>QVVSQGWKYFKGNFYYFSLIPKTWYSAEQFCVSRNSHLTSVTSESEQEFLYKTAGGLIYWIGLTKAGMEGDWSWVDDTPFNKVQSARFWIPGEPNNAGNNEHCGNIKAPSLQAWNDAPCDKTFLFICKRPYVPSEP[4x]

Langerhans cells are characterized by the presence of langerin (CD207), a C-type lectin that can act as a pathogen receptor by binding to surface glycoconjugates of microorganisms. Langerin has an extracellular region that contains (1) a C-type carbohydrate-recognition domain (CRD) that binds sugars and (2) a neck region that mediates the formation of trimers. As in other C-type lectins, the CRD of langerin contains a conserved Ca2+ binding site that binds to carbohydrates. Here we report the identification of additional glycan ligands for langerin through screening of a microarray of bacterial lipopolysaccharides and high-resolution crystal structures of the langerin CRD bound to carbohydrates representing a spectrum of ligands.

Electron density for both sugars in the disaccharide is seen in two copies of the CRD, whereas only a single-mannose residue is observed in the other two. The disaccharide adopts the preferred conformation seen in other crystal structures. Unlike in the Man4 and Man5 structures, two orientations for the mannose bound in the Ca2+ site are observed, each at approximately 50% occupancy, in each of the four crystallographically independent copies of the Man2–CRD complex. One orientation is the same as that observed for the terminal mannose residue in the Man4 and Man5 structures, in which the 3-OH group coordinates Ca2+ and forms hydrogen bonds with Glu293 and Asn307, the 4-OH group coordinates Ca2+ and forms hydrogen bonds with Glu285 and Asn287, and the 2-OH group forms a hydrogen bond with Lys299. When the full disaccharide is visible in this orientation, the residue at the nonreducing end is in the primary binding site, and the 4-C of the mannose residue at the reducing end packs against Ala289. In the second orientation, the sugar ring is rotated about an axis perpendicular to the C3–C4 bond, so that the partners of the 3-OH and 4-OH groups are reversed, and the oxygen attached to the anomeric carbon forms a hydrogen bond with Lys299. In this orientation, when the disaccharide is visible, the reducing end residue is the one ligated to Ca2+, and the second residue does not contact the protein. In the first conformation, the chain can be readily extended from the reducing end. At the other end of the disaccharide, glycans in which the 6 position of the mannose bound at the Ca2+ site is on the reducing side of an α1–6-linked sugar can also be accommodated, since the 6-OH group of this mannose points away from the protein surface. In the alternative conformation, the 6 position of the nonreducing mannose is away from the protein surface, allowing elongation from this end, and an α1–3 linkage of the Ca2+-ligated mannose to GalNAc, as in polysaccharide 44, could also be accommodated.>METTVLVTFEQRLTTGDVGKLSRLIGAVIPIPYRHHLLGSSQVGLDAVVKDKTRDYSRMRARMREMTLTIMRRVEGNQMILGVPTHGQCYTIRNTGPVSWEKGDVLTTLPPVFSGEVTGLVSVSDWDLVLPWIVPMALATEINQRMMMLALLSLDRSHEEVRAATAQLRVVRYRDATLTLPEITIDDTVLIDMRNVCISLSMIANLSSEVTLAYVRKLALEDSNMLLMKCQEILGRRMPQVGVGAGSSGDRNDPPARSRTNYNITPTEELNKLTALFVMIRQITDVISEQPAFLVCDVSPDDKSALCIYKG[10x];>MSARGRAAGDDGRQAELMATLGFVRLSKSSVGKVKKFLNNLYDLKSINLCRHPRVIAECRGTDLSRETQLYNEMVLWLRYHEKLTARRPGHLPLLTRIRQDYDKLFGFVAARPELCGFDGLTEVNVFDDAVYGDDYVPRVDVFLRGLEDLARCLCAQGPDKPARAVIMGFINMRAEEVNRLMDNVRDAAERVLVYEVLDVRDPLNEDPSVLVHNRLVYLCRLAYAISKSWQTLSHMCLDRINSLRRRLILAFHDRPAFARVYARNALERPVDGTTAYNLLRRLEEDFLLFRNALRWGDPDWGLESELESEGDNSDAGSDLDLEDEEDDDDGGGPGGHDDESGGNRTPDPGMSLHDDTGIANTCLIGGDDEDCGGGSGRCLEFDPDSERCLGVKMVNGRALRWWNPTGIMVDNEAAVWIDEHGRVMDKPPPKELRKASSDDGGNKKNPPPKKNVTPPVSGSNSVGGGVQTPSTASGKRTGKKKEGGGGYLLRSRSTDDDEVRKMKKDGTIDDRADRELKMALQKARESTADSDLSTILPRTEPLRKVAFVGDPVAAFGDTVRTTSSSKGFDDGPFTTQGASVLLPPPLGGPGSTLTLPPDLPDLSGVLADEDVQDSRYGKIPKSRTKKHPTFPENYKQRPPPHNKDDEYYWDETGDNMPVGEDGGGVLEDLRKGLEGIDLKTGGGGSLQPPLSQQFAGSPFAGSDGDGGGLVKKSSSSH[8x];>[16x]MGENWTATELLPKLDVPIDLLTHIKLSVGEEMFNNFRLYYGDDPERYNLSFEAIFGTYCNKIEWVTFLGTALATAAHAIMFHDLNKMTTGKMLFYIQVPRVATGAGIPTSRQTTVMVSKYSEKSPITIPFEISAACLTHLKETFEDTLLDKLLNADAVNTVLRAVKNTADAMERGLIDTFLRVLLRHAPPCFVLRTLMEHGTIARRMATRVQRANIAQGFKSKMLATIFLLDRSRDRGQLTRYLDMLTDCVTESILDNPETYTVGGGERLAGVIVSTHTVVQALLNALGGSIRRTGVKTPASYGKFVLSKENAVTAIAHHAIMADFSQHADRIQQSSQKDLPESQFLDQRLTFTETQMDVLKVGERLVALEHLRKVYKNTDVQDPLERDVELTFYFPVGLHVPSGRAYSTAENKIKLVDTAENQLPTTVYFYNKDRIPQRISHAEALKTLCHPAIHDAGPCLEAFAQAGPPQGDDRVRALCRREFVREHMAHATRRLVHFYQARIDPPRTANEAKHDFSTKEFAKVDNYLLFTELHPFFDFCFHTENGQVRPLCTPRIMVGNLPEALAPADFHDLRAKQALELTKVRAPEGHEATLQVLRASLTDHQYPELFYLIESLIHGDPAAFETGIELVTRCVNNYWRQRGLLAFANSYDMVRLIATRLGDGAVVPAAYTHYRNLLSITRFVARTCELTGLNGRLCDEPLLAYVSALHDPRLWPPFV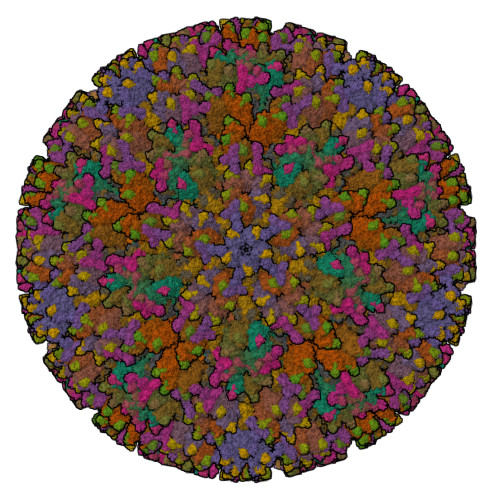QALPRNANLVRVVADDVPLDAAHIEERNPGTSDVARMIAMDQAEPLFVDARRTSDEEMVAQKVYYLCLVPAVLNNHACGAGLNLKHLLVKLFYTKFFLTADPDSLTAGEEALTNNPLLAALVRDVATDENVTANQAAEELFHLVAHVPENAQMLEIRAALDPAQRHGAPSAGFESLQHVLYNGFCMTTVPKLLQEYLTVIPFHRFYSDPGLAATANHDIRVFLNDFPQYQRCDGGFPLSPIFAHEYHHWHRTPFSCYSAACAHTLESVLTLAIMHHKMSPVSIAALSRMGLHPGFALTVVRTDTFETDTLLYSTKASTAVIINTPIVTKEDRDINTVFHVSQNINTVEMGLGYGATTCTAHLRRVRSDMGSRMQDLFQVFPMHVYRNEDVDAWVRQATGARRTEVLDSEAISILTFGRKTDKGGPALLHGQRATCEVILTPVSADLEFFRYPNNPRGRSSSMLGVDPYDEDAALATLYDHTSPDPQTFVSTNNPWGSQRGSLGDVIYNTRNREKLGHNPSFYSPCAQFFTTDDIINANKTLFKTVEEYLNRSQDCIHGETDLQYICVEGTNSIVEKPCRFLQEALTQHTGTTQALMESQLKGTSKLGLDETHYGNYSIGETIPLQQSILFNS;>MSTNVSSAASGGGSSGGSSGASSGGGGGGSGGSSKKEEERRKQFGANVLNLAPAMVAQPVISTMIPKYMKMGGHEDKLAYQLDLLRMLSIAKKATVIQ[16x];>[5x]MANVSSFGPMKREVMEFDPEDPYKVSKMRKLERSIAKGYVYGADHQAITARFFVRESLGEVEQKNLGVLMFRLDTGIEMPSTVLVSLFFLSMVAENVSAATKNTLAAIYGREGEAIRTWLRDGAWRLHRVVHPLGCTNSITPGATCLITCSMRGHSYNMLKTEIYPLLVPKEIYLDLDGESTDEIRFVYFVITYDYNSDRQGRPSAFVVVSRITHRHTLINVLRYRFRVSRFHFLNNSISGYGPSTGCLGTLQRLGWFCSRDSRSGIVASRAGQLSVVKLEKFYVDVGPLVEFA>VRSSSRTPSDMPVAHVVANPQAEGQLQWKNAGANALLANGVELRDNQLVVPSEGLYLIYSQVLFSGQGCPSTHVLLTHTISRIAVSYQTPVNLLSAIRSPCQRETPEGAEANPWYEPIYLGGVFQLEPGDRLSAEI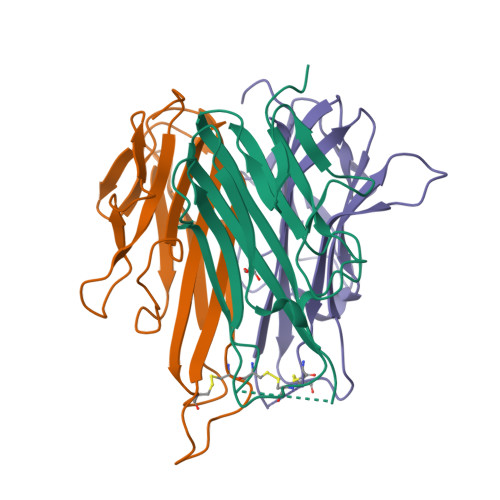NRPDYLDFASTGQVYFGIIAL[3x]> MSYQNLVSEAGLTQKHLIHGDKELFQHEMKTIFARNWLFLTHDSLIPSPGDYVTAKMGLDEVIVSRQNDGSVRAFLNVCRHRGKTIVHAEAGNAKGFVCNYHGWGYGTNGELQSVPFEKELYGDAIKKKCLGLKEVPRIESFHGFIYGCFDAEAPPLIDYLGDAAWYMEPTFKHSGGLELVGPPGKVVVKANWKTFAENFVGDIYHVGWTHASILRVGQSVFTPLAGNAMLPPEGSGLQMTSKYGSGMSLMWDYYAGNHSADLVPDLMAFGGAKQEKLAKEIGDVRARIYRSHLNGTIFPNNSFLTGSAAFKVWNPIDENTTEVWTYAFVEKDMPEDLKRRLADAVQRTVGPGGYWESDDNDNMETLSQNAKKYQSSNSDLIASLGFGKDVYGDECYPGVVGPSGASETSYRGFYRAYQAHISSSNWAEFENASRNWHTELTKT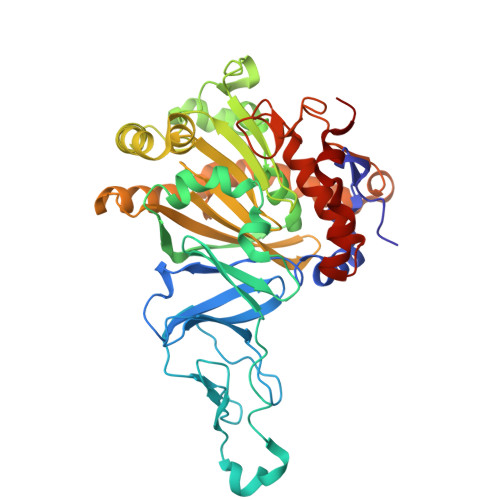TD> TETTSFSITKFSPDQQNLIFQGDGYTTKGKLTLTKAVKSTVGRALYSTPIHIWDRDTGNVANFVTSFTFV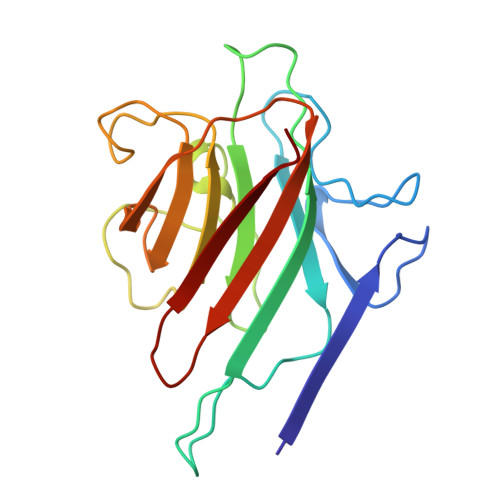IDAPSSYNVADGFTFFIAPVDTKPQTGGGYLGVFNSKEYDKTSQTVAVEFDTFYNAAWDPSNKERHIGIDVNSIKSVNTKSWNLQNGERANVVIAFNAATNVLTVTLTYPN> MKTIFTKKQTEELLNDISIEKQKELFNSMHDFRSQHAKEARIPGWSDKYNKLEKKMLSDFEEVTGIKYDTLESELIWDNLSNKFLYNS

AcrIIA28 is classified as an anti-CRISPR protein renowned for its capacity to impede the DNA cleavage activity inherent to the Cas9 enzyme. Our current study reveals that AcrIIA28 is a metalloprotein that contains Zn2+ and abolishes the cleavage activity of Cas9 only from Streptococcus pyrogen (SpyCas9) by directly interacting with the REC3 domain of SpyCas9. Furthermore, we demonstrate that the AcrIIA28 interaction prevents the target DNA from being loaded onto Cas9. Finally, based on our observations, we concluded that AcrIIA28 can inhibit the DNA-cleavage activity of SpyCas9 by directly interacting with the REC3 domain, which then can prevent the target DNA from being loaded into the Cas9 active site.

Finally, the 1.45 Å high-resolution structure of AcrIIA28 was determined, and the final structural model was refined to Rwork = 19.75% and Rfree= 20.36%. The crystal belonged to space group P41212 and contained a single molecule in the asymmetric unit (ASU). The final structural model covered most of AcrIIA28 (residues M1 to Y86), excluding the last two C-terminal amino acids due to unclear electron density. The structure of AcrIIA28 consisted of four α-helices (α1–α4). Two major long helices in the centre (α2 and α3) is covered by two short helices from N- and C-terminal parts (α1 and α4). B-factor analysis highlighted high rigidity, with low B-factor values (average 25.3 Å) for most of the structure, except the α3 region (average 48.2 Å), underscoring the rigid conformation of the AcrIIA28 protein in solution. In addition, the other selected proteins also exhibited low Z-scores (around 5.9–5.6) and sequence identity (2–12%), indicating that the AcrIIA28 structure is novel, whose fold has not been reported previously. During the structural refinement step, we found a big round-shape electron density, which exhibited a typical metal ion density, around the α3–α4 connecting loop region of AcrIIA28. This metal ion density was coordinated by oxygens from the main chain of E39, I42 and G44. To reveal the identity of this metal ion, we used inductively coupled plasma mass spectrometry (ICP-MS). This analysis indicated that Zn2+ was the metal ion, with a detected concentration of 105.3 ppb (μg/kg).> MMKHEVVALKKKSIGTSVLRREDTRLLTGRGRYIADLVLSGMLHVASLRSPFAHARIVSIDVADAQALPGVELVWCGADVAELSQGIVATMQVEGFQTTIQPLLANGVTRFVGEIVAVVVASSRAIAEDAAQLIQVEYEELPAVTGIEAALEGEARANDTLAGNVVSRTSRARDELAPIFASSAGVVRGQFSCGRVSACPMETRGAVAQYEWTTQQLILWTATQMPSFVRTMVAMFCAIPEHLIEVRVPDVGGGFGQKAHLHPEELLVCLLSRALGRPVRWIEDRQENFLGATHAKQQRNEMGLAFDGDGRFLALENRSITDGGAYNNLPWTQLVESHVGNAVILGVYKVPAVSEESIAVATNKCPIGAYRGVGFTAGQIARETLIDRAARQLGLSPFEIRRRNVVMPEDFPFTNRLGQTHREGTYLQTINLLEEMVNPEAFRQRQAEARARGKYLGLGVSVFNEVTGTGTRTLSFLGTPTTTHDSATVRIDPTGKVTVTTSLASSGQGHETTLAQIAADVLGVPASDVVIQAGSTKNTYGFGAYASRGAVIGAGSIGRAASIVRERVKQLAGHLLEAASEDIVIEDGLVHVAGVPAKGMPFAEVVGAAYFADATHPPGFDATLEATATYDPSDLVLANGGHAAIVEIDASTYATRVTDFFAVEDCGTMINPMIVEGQIRGGIAQAIGQT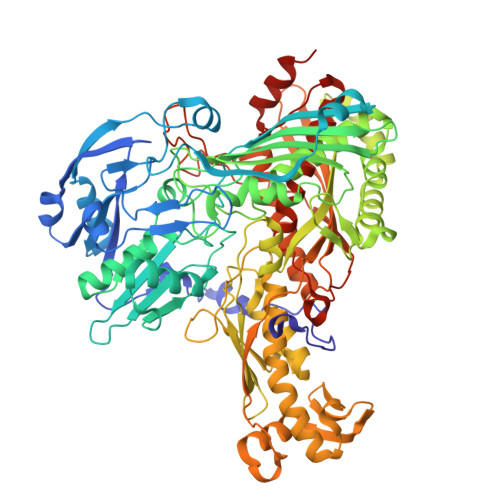LLEEVIYDDFGQLVTTTLMDYLIPTTLDVPDIRIRHLETPSPLVPGGIKGMGESAMISAPAAVVAAVNDALAHLEVVIETVPITPERIFRSIQERPMQ>[2x]GGPSFPEPKVVRSQGGLLSLKLSATPTPLAIAGQRATLLTYGGSFPGPTLRVRPRDTVRLTLENRLPEPTNLHWHGLPISPKVDDPFLEIPPGESWTYEFTVPKELAGTFWYHPHLHGRVAPQLFAGLLGALVVESSLDAIPELREAEEHLLVLKDLALQGGRPAPHTPMDWMNGKEGDLVLVNGALRPTLVAQKATLRLRLLNASNARYYRLALQDHPLYLIAADGGFLEEPLEV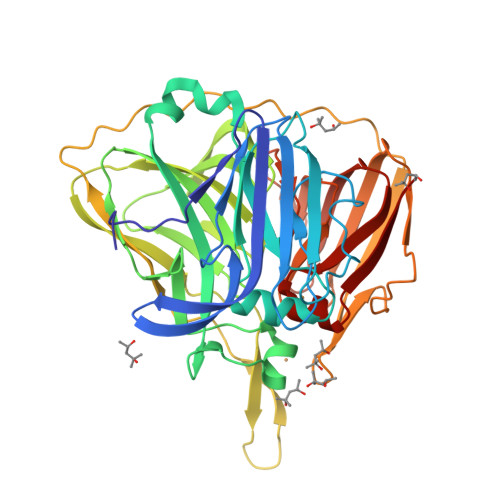SELLLAPGERAEVLVRLRKEGRFLLQALPYDRGAMGMMDMGGMAHAMPQGPSRPETLLYLIAPKNPKPLPLPKALSPFPTLPAPVVTRRLVLTEDMMAARFFINGQVFDHRRVDLKGQAQTVEVWEVENQGDMDHPFHLHVHPFQVLSVGGRPFPYRAWKDVVNLKAGEVARLLVPLREKGRTVFHCHIVEHEDRGMMGVLEVG>MRLSGSDGRRLTYRTSPRVRASLLLLGAIVLLVYF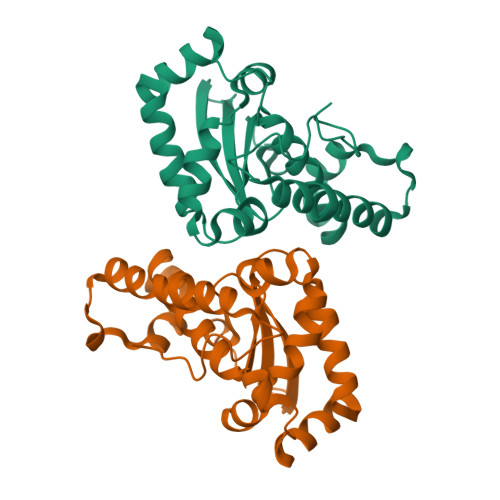AETLFVVCRGSMDSRAVRHAIPSGKGLRAKPFVPSRSGVAPSSGLRMTLPYGLEALEPVISAATVDFHYNKHHQGYIQKLLDATGLPESRINLKSLVTLGPDRAGENVFNAAGQIYNHNMYWLSMVPTSGSGRHVPPRLLKLIRARWGNVDEMKENFMRKATALFGSGWIWLVWDTRERRLDLVGTKDAHSPLSEDAGKIPLFTCDVWEHAYYLDYQHDRAAYLTRWWSLINWEFADSNLPSDIE[2x]In this study, we focus on a resistance gene cph, which encodes a phosphotransferase (Cph) that confers resistance to the antituberculosis drug capreomycin (CMN). To confirm whether proteins in cluster I also confer resistance to CMN, three proteins, Cph001 from Streptosporangium roseum (accession number: WP_012891209), Cph002 from Streptomyces sp. SID8364 (MYT78782), and Cph003 from Streptomyces filamentosus NRRL15998 (EWS93654), were selected for disk diffusion assays. The polypeptide chain of Cph001 is folded into two domains, an N-terminal lobe domain (Met1–Gly97) and a C-terminal domain (Ala98–Arg286). The C-terminal domain further divided into a core subdomain (Ala98–Ala140 and Thr182–Ser246) and an α-helical subdomain (Pro141–Ile181 and Asp247–Arg286).

We then performed mutagenesis on the codons coding for the conserved catalytic residue Asp189 to generate the Cph001D189A and Cph001D189N variants. Activity assays revealed that both mutations resulted in complete loss of phosphotransferase activity supporting that Asp189 in Cph001 plays a critical role for catalysis. Degradation bands were observed on the SDS-PAGE for the wild-type Cph001 after a week of storage at 4 °C. This might be the reason why the wild-type Cph001 could not be crystallized. After multiple attempts to obtain the crystals of the wild-type Cph001, we switched to focus on the Cph001D189N variant, which is more stable than the wild-type and can be crystallized at 4 °C. Crystals of Cph001D189N were successfully obtained in a week and the diffraction data were collected at National Synchrotron Radiation Research Center (NSRRC) on beamlines 15A, 05A, or 07A. The molecular packing of Cph001D189N belongs to the orthorhombic space group P212121. Two polypeptide chains were found and built in the asymmetric unit. The final model of Cph001D189N was refined to a resolution of 2.3 Å. In every Cph001 structures, including apo and complex forms, the two polypeptide chains within the asymmetric unit adopt distinct conformations: an open form and a closed form. The two forms implicate conformational changes during enzyme catalysis. The closed form reveals that the α-helical subdomain moves closer to the N-terminal lobe domain when compared to the open form.

>[2x]MGILQANRVLLSRLLPGVEPEGLTVRHGQFHQVVIASDRVVCLPRTAAAAARLPRRAAVMRVLAGLDLGCRTPRPLCEGSAEGAVELPFLVLSRVPGAPLEADALEDSKVAEVVAAQYVTLLSGLASAGADEKVRAALPAPQGRWRQFAADVRAELFPLMSDGGCRQAERELAALDSLPDITEAVVHGNLGAENVLWVRDDGLPRLSGVIDWDEVSIGDPAEDLAAIGAGYGKDFLDQVLTLGGWSDRRMATRIATIRATFALQQALSACRDGDEEELADGLTGYR> TRTVFVGNHPVSETEAYIAQRFCDNRIVSSKYTLWNFLPKNLFEQFRRIANFYFLIIFLVEVTVDTPTSPVTSGLPLFFVITVTAIKQGYEDWLRHRADNEVNKSTVYIIENAKRVRKESEKIKVGDVVEVQADETFPCDLILLSSCTTDGTCYVTTASLDGESNCKTHYAVRDTIALCTAESIDTLRAAIECEQPQPDLYKFVGRINIYSNSLEAVARSLGPENLLLKGATLKNTEKIYGVAVYTGMETKMALNYQGKSQKRSAVEKSINAFLIVYLFILLTKAAVCTTLKYVWQSTPYNDEPWYNQKTQKERETLKVLKMFTDFLSFMVLFNFIIPVSMYVTVEMQKFLGSFFISWDKDFYDEEINEGALVNTSDLNEELGQVDYVFTDKTGTLTENSMEFIECCIDGHKYKGVTQEVDGLSQTDGTLTYFDKVDKNREELFLRALCLCHTVEIKTNDAVDGATESAELTYISSSPDEIALVKGAKRYGFTFLGNRNGYMRVENQRKEIEEYELLHTLNFDAVRRRMSVIVKTQEGDILLFCKGADSAVFPRVQNHEIELTKVHVERNAMDGYRTLCVAFKEIAPDDYERINRQLIEAKMALQDREEKMEKVFDDIETNMNLIGATAVEDKLQDQAAETIEALHAAGLKVWVLTGDKMETAKSTCYACRLFQTNTELLELTTKTIEESERKEDRLHELLIEYRKKLLHEFPKSTRSFKKAWTEHQEYGLIIDGSTLSLILNSSQDSSSNNYKSIFLQICMKCTAVLCCRMAPLQKAQIVRMVKNLKGSPITLSIGDGANDVSMILESHVGIGIKGKEGRQAARNSDYSVPKFKHLKKLLLAHGHLYYVRIAHLVQYFFYKNLCFILPQFLYQFFCGFSQQPLYDAAYLTMYNICFTSLPILAYSLLEQHINIDTLTSDPRLYMKISGNAMLQLGPFLYWTFLAAFEGTVFFFGTYFLFQTASLEENGKVYGNWTFGTIVFTVLVFTVTLKLALDTRFWTWINHFVIWGSLAFYVFFSFFWGGIIWPFLKQQRMYFVFAQMLSSVSTWLAIILLIFISLFPEILLIVLKNVR;> RPDNTAFKQQRLPAWQPILTAGTVLPIFFIIGLIFIPIGIGIFVTSNNIREIEIDYTGTEPSSPCNKCLSPDVTPCFCTINFTLEKSFEGNVFMYYGLSNFYQNHRRYVKSRDDSQLNGDSSALLNPSKECEPYRRNEDKPIAPCGAIMNSMFNDTLELFLIGQDSYPIPIALKKKGIAWWTDKNVKFRNPPGGDNLEERFKGTTKPVNWLKPVYMLDSDPDNNGFINEDFIVWMRTAALPTFRKLYRLIERKSDLHPTLPAGRYWLNVTYNYPVHYFDGRKRMILSTISWMGGKNPFLGIAYIAVGSISFLLGVVLLVINHKY

Closely related P4-ATPases, ATP11A and ATP11C, act as major phospholipid flippases in the plasma membrane of mammalian cells, with strict substrate specificity for phosphatidylserine (PS) and phosphatidylethanolamine (PE), but not for phosphatidylcholine (PC), thereby contributing to the asymmetric distribution of PS and PE across bilayers. In contrast, flippases, also known as P4-ATPases, translocate their specific substrate phospholipid from exoplasmic to the cytosolic leaflet of the bilayer coupled with ATP hydrolysis. Most mammalian P4-ATPases, except ATP9A and ATP9B, require an accessory subunit, CDC50A, for their proper localization and functional expression in the plasma membrane. A previously reported disease-associated Q84E mutation in ATP11A confers the ability to flip PC, implicating the involvement of this conserved residue in substrate specificity.

The cryo-EM structure of ATP11C Q79E mutant in the PC-occluded E2-Pi state revealed a PC molecule in a reshaped binding pocket. Due to the Q79E mutation and associated conformational changes in its surrounding residues, including Ser91and Asn352, the binding pocket has additional space to accommodate the bulky choline headgroup. Arrangement of TM helices, especially TM1, TM2, TM4 and TM6 that form the phospholipid-binding pocket, is unchanged between PS-occluded WT and PC-occluded Q79E mutant, suggesting a preserved gating mechanism between them. In contrast, PC, with three methyl groups at its terminus, cannot form hydrogen bonds with surrounding hydrophilic side chains. The nitrogen of the quaternary amine in PC is located more than 4 Å from the carboxyl group of Q79E, suggesting that it does not engage in strong electrostatic interactions. This observation refutes an intuitive hypothesis that the Gln to Glu mutation enhances PC binding due to increased electrostatic interaction, as the nitrogen on the PC quaternary amine is presumed to be positively charged at a neutral pH. A detailed comparison of the WT and Q79E mutant structures revealed that the respective side chain rotamer conformations (i.e., Q79 in WT and E79 in Q79E mutant) are different, each rotating approximately 90° relative to one another. In contrast, the Ser91 side chain in the Q79E mutant faces the opposite direction, and it appears to stabilize its conformation by forming a hydrogen bond with the carboxyl of Q79E (see arrow for the displacement of side chains). Due to the rotation of Q79E relative to Gln79 in WT, Asn352 makes a hydrogen bond with Q79E, thus the side chain conformation of Asn352 also slightly changes compared to that in WT. While the WT binding pocket and PS-occluded structure of the Q79E mutant are ideally shaped to fit the PS head group, the PC-occluded structure of the Q79E mutant shows a slightly widened pocket, particularly due to the changes in Ser91 and Asn352 side chain conformations that directly contact PC head group.(5R,7R,8S,9S,10R)-7-(HYDROXYMETHYL)-3-(4-METHOXYPHENYL)-1,6-DIOXA-2-AZASPIRO[4.5]DEC-2-ENE-8,9,10-TRIOL 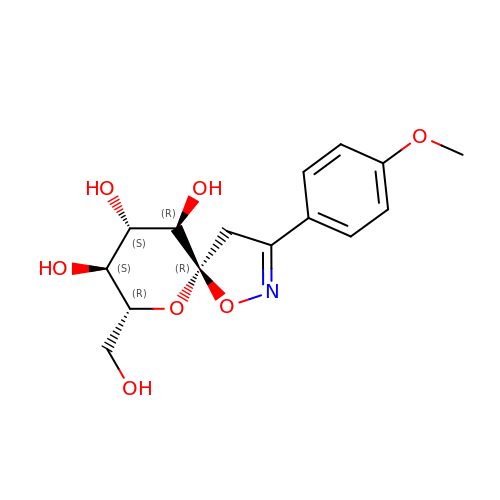| C15 H19 N O7 | SCPKUJWXPVROSY-UXXRCYHCSA-N ID30A-3 (or MASSIF-3) is a mini-focus (beam size 18 µm × 14 µm) highly intense (2.0 × 1013 photons s−1), fixed-energy (12.81 keV) beamline for macromolecular crystallography (MX) experiments at the European Synchrotron Radiation Facility (ESRF). MASSIF-3 is recommended for collecting diffraction data from single small crystals (≤15 µm in one dimension) or for experiments using serial methods.

In a second experiment, bovine trypsin purchased as lyophilized powder from Sigma (reference: T9201) was crystallized as follows: A solution of 40 mg ml−1 trypsin, 10 mg ml−1 benzamidine (Sigma B-6506) and 3 mM CaCl2 was mixed in a 1:1 ratio with reservoir solution [2 M (NH4)2SO4 in 100 mM Tris-HCl pH 8.5] at room temperature. Crystals appeared after a few days and were cryo-protected using 20% (w/v) glycerol. Diffraction data were then collected at 100 K using two different strategies: the first based on a strategy provided by EDNA/BEST, the second using a manually determined strategy optimized for data collection speed. While the ‘slow’ diffraction data set has been collected to show a standard data collection, the ‘fast’ diffraction data set has been collected to show the potential of the beamline. As can be seen in Table 2, the two data sets are of comparable quality (automatic processing using EDNAproc) with both giving clear structure solutions, requiring only little additional refinement (adding waters, benzamidine and other buffer molecules, adjusting side chains, etc.), using the ESRF automatic molecular replacement pipeline.

> MKTFIFLALLGAAVAFPVDDDDKIVGGYTCGANTVPYQVSLNSGYHFCGGSLINSQWVVSAAHCYKSGIQVRLGEDNINVVEGNEQFISASKSIVHPSYNSNTLNNDIMLIKLKSAASLNSRVASISLPTSCASAGTQCLISGWGNTKSSGTSYPDVLKCLKAPILSDSSCKSAYPGQITSNMFCAGYLEGGKDSCQGDSGGPVVCSGKLQGIVSWGSGCAQKNKPGVYTKVCNYVSWIKQTIASN N-(4-{[(2,4-diamino-7,8-dihydropyrido[3,2-d]pyrimidin-6-yl)methyl]amino}benzene-1-carbonyl)-L-glutamic 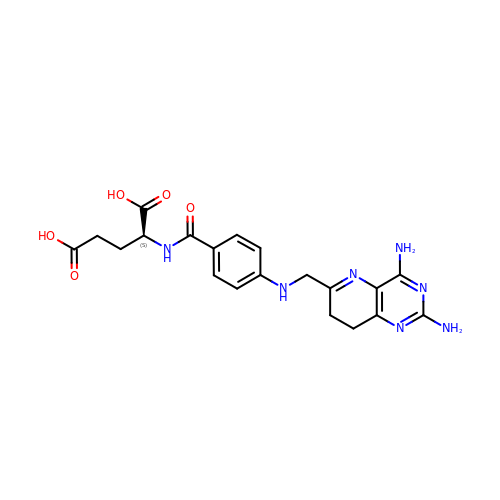acid | C20 H23 N7 O5 | QECVBNUHIUCZFO-AWEZNQCLSA-N> MNYNLSKYPDDVSRLFKPRPPLSYKRPTDYPYAKRQTNPNITGVANLLSTSLKHYMEEFPEGSPNNHLQRYEDIKLSKIKNAQLLDRRLQNWNPNVDPHIKDTDPYRTIFIGRLPYDLDEIELQKYFVKFGEIEKIRIVKDKITQKSKGYAFIVFKDPISSKMAFKEIGVHRGIQIKDRICIVDIERGRTVKYFKPRRLGGGLGGRGYSNRDSRLPGRFASASTSNPAERNYAPRLPRRETSSSAYSADRYGSSTLDARYRGNRPLLSAATPTAAVTSVYKSRNSRTRESQPAPKEAPDY;> MTRYYCEYCHSYLTHDTLSVRKSHLVGKNHLRITADYYRNKARDIINKHNHKRRHIGKRGRKERENSSQNETLKVTCLSNKEKRHIMHVKKMNQKELAQTSIDTLKLLYDGSPGYSKVFVDANRFDIGDLVKASKLPQRANEKSAHHSFKQTSRSRDETCESNPFPRLNNPKKLEPPKILSQWSNTIPKTSIFYSVDILQTTIKESKKRMHSDGIRKPSSANGYKRRRYGN;> MSALYFQNLPSRPANKENYTRLLLKHINPNNKYAINPSLPLPHNKLQISSQPLMLLDDQMGLLEVSISRSSKMTNQAFLTFVTQEEADRFLEKYTTTALKVQGRKVRMGKARTNSLLGLSIEMQKKKGNDETYNLDIKKVLKARKLKRKLRSDDICAKKFRLKRQIRRLKHKLRSRKVEEAEIDRIVKEFETRRLENMKSQQENLKQSQKPLKRAKVSNTMENPPNKVLLIQNLPSGTTEQLLSQILGNEALVEIRLVSVRNLAFVEYETVADATKIKNQLGSTYKLQNNDVTIGFAKGRRIPGLINPWKRRWKKNFIAVSAANRFKKISSSGALDYDIPTTASENLYFQ;> MDKYTALIHDENFSTLTLNVSRYPKSLAYWEKLLNYIVKASAPICKSTEPQLLKLIRCTYSSMLNEFPYLENYYIDFALLEYKLGNVSMSHKIFQRGLQAFNQRSLLLWTSYLKFCNNVISHQKQLFKKYETAEEYVGLHFFSGEFWDLYLEQISSRCTSSKKYWNVLRKILEIPLHSFSKFYALWLQRIDDIMDLKQLSQLTSKDELLKKLKIDINYSGRKGPYLQDAKKKLKKITKEMYMVVQYQVLEIYSIFESKIYINYYTSPETLVSSDEIETWIKYLDYTITLQTDSLTHLNFQRALLPLAHYDLVWIKYSKWLINSKNDLLGAKNVLLMGLKFSLKKTEIIKLLYSVICKLNEYVLLRNLLEKIESSYSDNVENVDDFEIFWDYLQFKTFCQNSLYSSRYSDSQSNGLLNKELFDKVWKRLSCKEKKSGQEILLNNLVQFYSKDTVEFVEKNIFQKIIEFGWEYYLQNGMFWNCYCRLIYFDTSRSYLDKRQYIVRKIWPQIDKKFAQSVLPSLTEFCESYFPEEMDTLEEMFTEEP;> MPDETNFTIEDIEPRPDALRGLDTQFLQDNTALVQAYRGLDWSDISSLTQMVDVIEQTVVKYGNPNDSIKLALETILWQILRKYPLLFGFWKRFATIEYQLFGLKKSIAVLATSVKWFPTSLELWCDYLNVLCVNNPNETDFIRNNFEIAKDLIGKQFLSHPFWDKFIEFEVGQKNWHNVQRIYEYIIEVPLHQYARFFTSYKKFLNEKNLKTTRNIDIVLRKTQTTVNEIWQFESKIKQPFFNLGQVLNDDLENWSRYLKFVTDPSKSLDKEFVMSVFDRCLIPCLYHENTWMMYIKWLTKKNISDEVVVDIYQKANTFLPLDFKTLRYDFLRFLKRKYRSNNTLFNNIFNETVSRYLKIWPNDILLMTEYLCMLKRHSFKNSLDQSPKEILEKQTSFTKILETSITNYINNQIDAKVHLQTLINDKNLSIVVVELIKTTWLVLKNNMQTRKYFNLYQKNILIKNSVPFWLTYYKFEKSNVNFTKLNKFIRELGVEIYLPTTVMNDILTDYKTFYLTHSNIVTYESSIIDSNTFDPILYPELKMSNPKYDPVLNTTANVDWHKKTEWKEAGHIGITTERPQISNSIIECNSGTLIQKPISLPNFRNLEKINQVKINDLYTEEFLKEGK;> MSYKQTTYYPSRGNLVRNDSSPYTNTISSETNNSSTSVLSLQGASNVSLGTTGNQLYMGDLDPTWDKNTVRQIWASLGEANINVRMMWNNTLNNGSRSSMGPKNNQGYCFVDFPSSTHAANALLKNGMLIPNFPNKKLKLNWATSSYSNSNNSLNNVKSGNNCSIFVGDLAPNVTESQLFELFINRYASTSHAKIVHDQVTGMSKGYGFVKFTNSDEQQLALSEMQGVFLNGRAIKVGPTSGQQQHVSGNNDYNRSSSSLNNENVDSRFLSKGQSFLSNGNNNMGFKRNHMSQFIYPVQQQPSLNHFTDPNNTTVFIGGLSSLVTEDELRAYFQPFGTIVYVKIPVGKCCGFVQYVDRLSAEAAIAGMQGFPIANSRVRLSWGRSAKQTALLQQAMLSNSLQVQQQQPGLQQPNYGYIPSSTCEAPVLPDNNVSSTMLPGCQILNYSNPYANANGLGSNNFSFYSNNNATNTQATSLLADTSSMDLSGTGGQQVIMQGSEAVVNSTNAMLNRLEQGSNGFMFA;> MRPRRRGLAYHHTKPKGQLSQGHYPTTSNDGQRRKVGNSEAFQSFDIWKNLDRIRSTKKNAGQFIKGSLLILPMRTEDKQQFDECMDELHKYISKDILRCYPQKEQKDEGMLFYIVLKDFNILDSCFVLSVLLAFQKRLWMAPSEKSYFRVPKNINLTGSFYLPKNIETGRGHIITSYRREQPSSSIVEVGFNVVPDFQQFQVKACHVSKFMNELSNFFSQVEFGKCEANVINYFKREYNRTYSQISLALYELPLIGDGLFDIKSYISKTRPIIETSKAQMIKHISEMKAYNEISGLQGDQFPRQQRPLSNSPSSNSISSSQTIEAGATSYQTQPQRHAVNKPSNVLNSSNRHSGPKTFEDGRYSEGNKPGFMTQDEIKQHCIGTIKASMDAVKKKSSYQILKTYVRCPRQNYIDIVYQNLNDLRSKTNCNIVVLNLNNLHESQMWLESLNTTNYTIFAQAPHPSTIRVISIGGVGEYIVKALELILNILEH;> MSTMSTPAAEQRKLVEQLMGRDFSFRHNRYSHQKRDLGLHDPKICKSYLVGECPYDLFQGTKQSLGKCPQMHLTKHKIQYEREVKQGKTFPEFEREYLAILSRFVNECNGQISVALQNLKHTAEERMKIQQVTEELDVLDVRIGLMGQEIDSLIRADEVSMGMLQSVKLQELISKRKEVAKRVRNITENVGQSAQQKLQVCEVCGAYLSRLDTDRRLADHFLGKIHLGYVKMREDYDRLMKNNRTTNASKTATTLPGRRFV;> MSIWKEAKDASGRIYYYNTLTKKSTWEKPKELISQEELLLRENGWKAAKTADGKVYYYNPTTRETSWTIPAFEKKVEPIAEQKHDTVSHAQVNGNRIALTAGEKQEPGRTINEEESQYANNSKLLNVRRRTKEEAEKEFITMLKENQVDSTWSFSRIISELGTRDPRYWMVDDDPLWKKEMFEKYLSNRSADQLLKEHNETSKFKEAFQKMLQNNSHIKYYTRWPTAKRLIADEPIYKHSVVNEKTKRQTFQDYIDTLIDTQKESKKKLK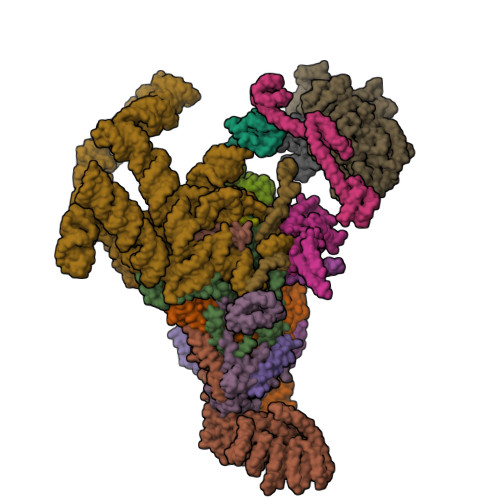TQALKELREYLNGIITTSSSETFITWQQLLNHYVFDKSKRYMANRHFKVLTHEDVLNEYLKIVNTIENDLQNKLNELRLRNYTRDRIARDNFKSLLREVPIKIKANTRWSDIYPHIKSDPRFLHMLGRNGSSCLDLFLDFVDEQRMYIFAQRSIAQQTLIDQNFEWNDADSDEITKQNIEKVLENDRKFDKVDKEDISLIVDGLIKQRNEKIQQKLQNERRILEQKKHYFWLLLQRTYTKTGKPKPSTWDLASKELGESLEYKALGDEDNIRRQIFEDFKPESSAPTAESATANLTLTASKKRHLTPAVELDY;> MSKIQVAHSSRLANLIDYKLRVLTQDGRVYIGQLMAFDKHMNLVLNECIEERVPKTQLDKLRPRKDSKDGTTLNIKVEKRVLGLTILRGEQILSTVVEDKPLLSKKERLVRDKKEKKQAQKQTKLRKEKEKKPGKIAKPNTANAKHTSSNSREIAQPSSSRYNGGNDNIGANRSRFNNEAPPQTRKFQPPPGFKRK;> MKLVNFLKKLRNEQVTIELKNGTTVWGTLQSVSPQMNAILTDVKLTLPQPRLNKLNSNGIAMASLYLTGGQQPTASDNIASLQYINIRGNTIRQIILPDSLNLDSLLVDQKQLNSLRRSGQIANDPSKKRRRDFGAPANKRPRRGL;> MSSQIIDRPKHELSRAELEELEEFEFKHGPMSLINDAMVTRTPVIISLRNNHKIIARVKAFDRHCNMVLENVKELWTEKKGKNVINRERFISKLFLRGDSVIVVLKTPVE;> MTMNGIPVKLLNEAQGHIVSLELTTGATYRGKLVESEDSMNVQLRDVIATEPQGAVTHMDQIFVRGSQIKFIVVPDLLKNAPLFKKNSSRPMPPIRGPKRR;> MSNKVKTKAMVPPINCIFNFLQQQTPVTIWLFEQIGIRIKGKIVGFDEFMNVVIDEAVEIPVNSADGKEDVEKGTPLGKILLKGDNITLITSAD;> MSESSDISAMQPVNPKPFLKGLVNHRVGVKLKFNSTEYRGTLVSTDNYFNLQLNEAEEFVAGVSHGTLGEIFIRCNNVLYIRELPN;> MVSTPELKKYMDKKILLNINGSRKVAGILRGYDIFLNVVLDDAMEINGEDPANNHQLGLQTVIRGNSIISLEALDAI;> MFNRKRRGDFDEDENYRDFRPRMPKRQRIPPVVQLCKEMMPDIRTIGESVKAFEDDIKFLSEAIMNEYGHEDYFNNALLSTLNAVVVEQPQKQAAIALLTMVVNSKNNVAGKSIINYFFEELQKWCKQTYNDEFKSTSNETGPWNKIKLILRFLSILSPMFLVDELINIYKSLFELSIELNNLDPGNRVPLSEAIYTNTLLNIPYLFFFNRNNDGLRTKVEELLAYVEQNYLVKTTDINLLREYNGEPPYEMVELVRVVLPNVKKALINNLEQLNELFPDWNHLLTPQTGDEGFNDALTLPSVDDLKSFVRLNKNFGSVDSMWKTPRYAFHVYLPNSAGNFETVVPISTYAGQLFNDIIIDLVESLEFNRKEVARQVITLDLFFKAGIFTEPGESIAQLIATYEENPLAPTFKIEDLAIETILGLIFKLPSVSQPFAYFYTLLVDICQNSPKAIAPVFGRAFRFFYSHLDSLDFELKLRYLDWFSIQMSNFNFSWKWNEWEDDSIKFGKYFYNPKVNFAKNLIQKELRLTSNFSEVEDSLPQEFTKYLDTSYIPRDQLINYYQSLFTGYTVEEDSVRKNDLYFRQEGVPMENTVRKILDYTHKANNSREVTELESILGELKNEYGSIISDFNRFVIILLVQAVTDSGSRSLSHANKYINDLKEDLKTIFAKIELDIETKEYIIIEAVLTFWNANPQTGFLVADAFKYAGLLTSRTIFTFIFNETGLKNNGLIEATAIEAVFRNLSQQISEENESGNNFEFVFERLCTIANSTIDLLDVNADEDIEIPKVNGEMDIDDIEDDKLDLKWKYFTVIGFIKSILRRYSHEYRELADKFIANIDNAIPHESTRRTISNWIQETKEV;> MSLEEFDEVKYDHSTKRLDTPSRYLLRKARRNPNGLQELRESMKSSTIYVGNLSFYTSEEQIYELFSKCGTIKRIIMGLDRFKFTPCGFCFIIYSCPDEALNALKYLSDTKLDEKTITIDLDPGFEDGRQFGRGKSGGQVSDELRFDFDASRGGFAIPFAERVGVPHSRFDNSSSQSNTNNYIPPPDAMGTFRPGFDEEREDDNYVPQ> MGIYSFWIFDRHCNCIFDREWTLASNSASGTINSKQNEEDAKLLYGMIFSLRSITQKLSKGSVKNDIRSISTGKYRVHTYCTASGLWFVLLSDFKQ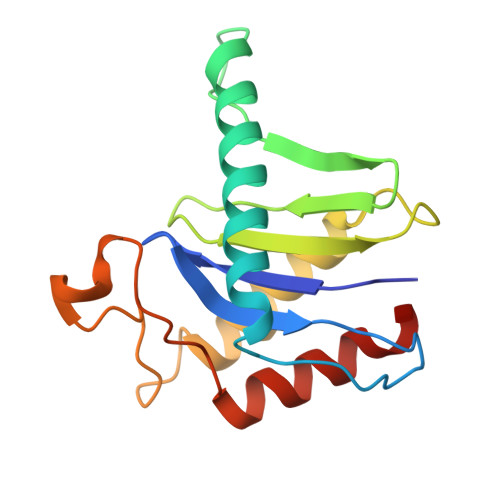QSYTQVLQYIYSHIYVKYVSNNLLSPYDFAENENEMRGQGTRKITNRNFISVLESFLAPMVNQ> MPKTTTFIQLVNKCLENIGERPVISFNNSVARKAADTVRDAITDVSYSYDWSWLTTSIIANSWINERADLGDVQSVKHVSYGSSSDGYRELTFTDERTFDAAKIYPGVGQVFTFNEYGGVRINPYPETVEEQVKYKFYVVKEATLPSVEIDVINIPDRFIQLITYNACTQLSISHLDDAQASQMWNSKYID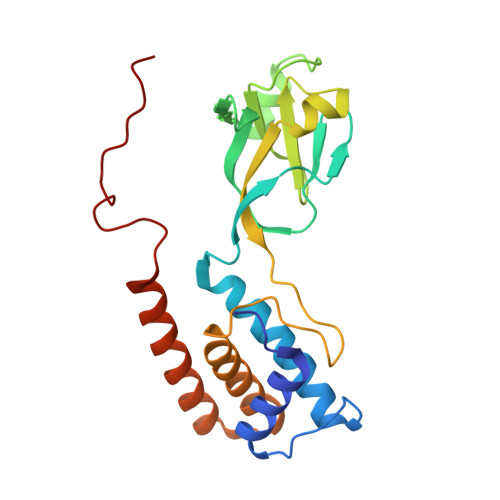QLSRLRARERNTTQSGANMFKFRGTR>[2x]SMGEIESYCNKELGPLPTKAPTLSKNVLDLFSLKGKVASVTGSSGGIGWAVAEAYAQAGADVAIWYNSHPADEKAEHLQKTYGVRSKAYKCNISDPKSVEETISQQEKDFGTIDVFVANAGVPWTEG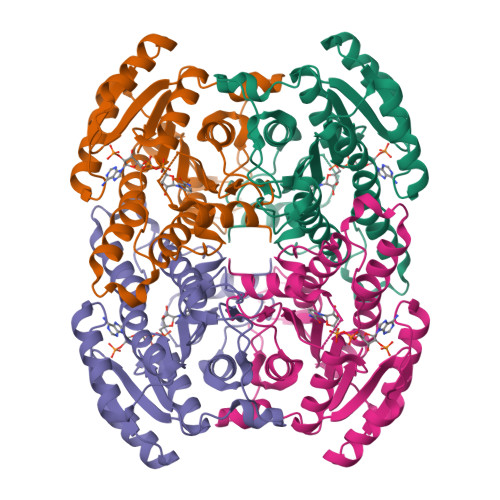PEINVDNYDSWNKIINLDLNGVYYCAHTVGKIFKKNGKGSLVITSSMSGTIVNVPQLQAAYNAAKAACTHLTKSLAVEWAPFARVNCVSPGYIATEISDFVEKDMKAKWWQLTPLGREGLAQELVGAYLYLASNASTYTTGANLAVDGGYTCP>[2x]NSPTLTRPPEGPKFPRVKNWELGSITYDTLCAQSQQDGPCTPRRCLG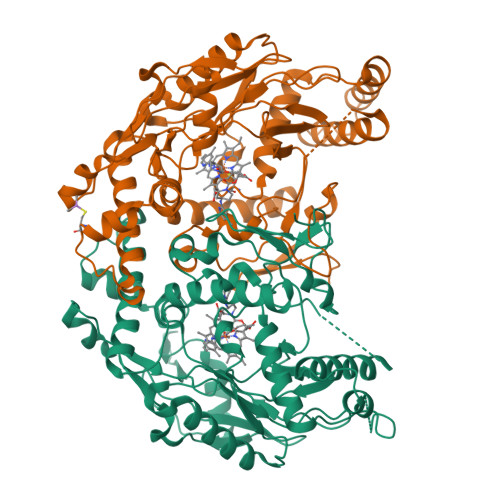SLVLPRKLQTRPSPGPPPAEQLLSQARDFINQYYSSIKRSGSQAHEERLQEVEAEVASTGTYHLRESELVFGAKQAWRNAPRCVGRIQWGKLQVFDARDCSSAQEMFTYICNHIKYATNRGNLRSAITVFPQRAPGRGDFRIWNSQLVRYAGYRQQDGSVRGDPANVEITELCIQHGWTPGNGRFDVLPLLLQAPDEAPELFVLPPELVLEVPLEHPTLEWFAALGLRWYALPAVSNMLLEIGGLEFSAAPFSGWYMSTEIGTRNLCDPHRYNILEDVAVCMDLDTRTTSSLWKDKAAVEINLAVLHSFQLAKVTIVDHHAATVSFMKHLDNEQKARGGCPADWAWIVPPISGSLTPVFHQEMVNYILSPAFRYQPDPWKGSAT>GUAXGUAC[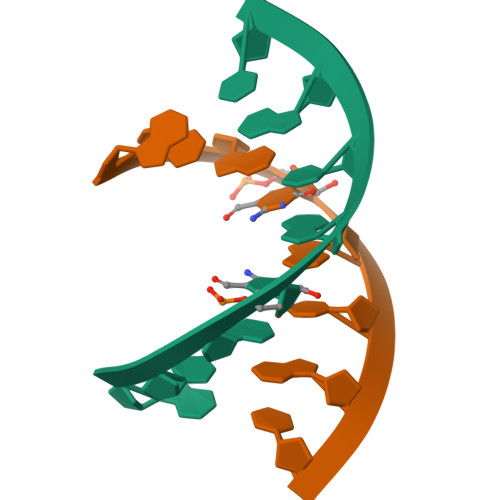6x]>MEGVKKIKNPSTVKDELLELMFRIYRSTNGKYPALEWVKRKPNPNDFNGFREVYEPFLKFRLSQEFDELYTYQKDNRIIGTIALVYKRIKEKGIWWVPEELMNEKVGLIEFFVVDPEFQGKGIGSTLLEFAVKRLRSLGKDPYVVTFPNLEAYSYYYMKKGFREIMRYKEFVILKFN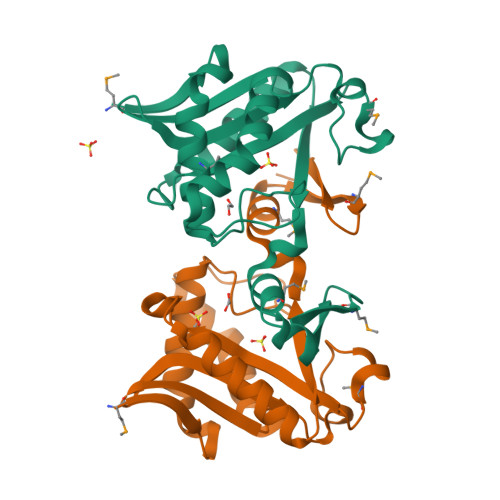HKKFQLEHHHHHH[2x]>MYTLIKLTSEYTSRAISFTSRNFVASEPTSIALKLTTCDFTTSFQNIMKQCVDYGHSFAFVDADDNIKAQILNIPYDAYENMHYGNIRETDPMFDLFGNLDSYTPDDKCLYVFAIGSEVTGKGLATKLLKKTIEESSSHGFKYIYGDCTNIISQNMFEKHGFETVGSVKYKGYQY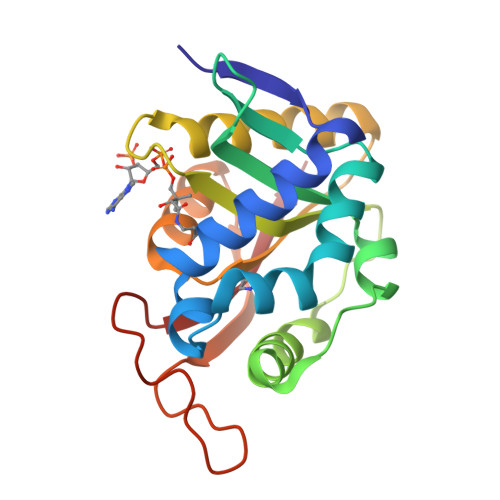GITKPFDSINCTEYIKRMVKTI[2x]>VAFGADAAKTTQEKFDALKEAGVFSGYPGTTDAKLGQDMTRAEFAKVLVKLFGLKEIHGQYSYKDKNYDAKNWAAPFIEAVTAEGLMQGKDLTKKIFDFNGKITVEEASKTLVTALKLEPVKDAQNKATDWAK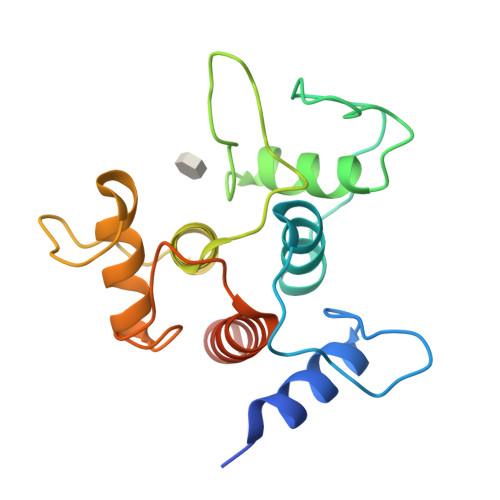GYFEAAVNAGLFSKDANPKANATRAQLVEAAFAADEMSKGSGSHHHHHH[2x]>MVRSSSRTPSDKPVAHVVANPQAEGQLQWLNRRANALLANGVELRDNQLVVPSEGLYLIYSQVLFKGQGCPSTHVLLTHTISRIAVSYQTKVNLLSAIKSPCQRETPEGAEAKPWYEPIYLGGVFQLEK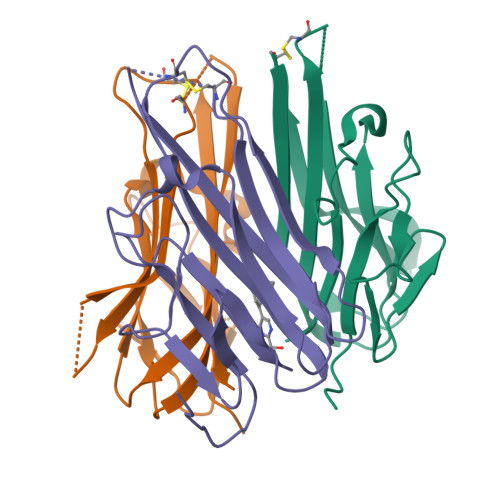GDRLSAEINRPDYLDFAESGQVYFGIIAL[3x]> MSQEQYTENLKVI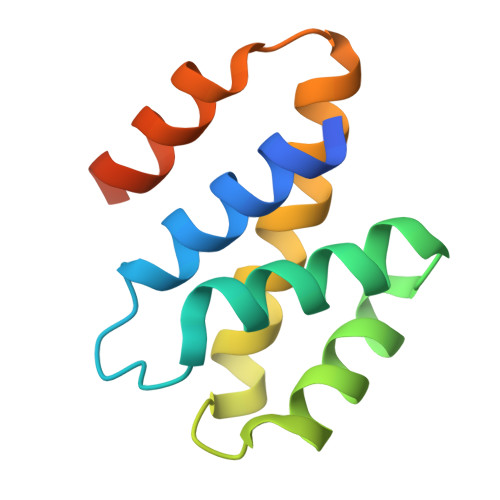VAEKLAGIPNFNEDIKYVAEYIVLLIVNGGTVESVVDELASLFDSVSRDTLANVVQTAFFALEALQQGESAENIVSKIRMMNAQSLGQSDI>MEGPAGYLRRADVAQLTQELGTAFFQQQQLPAAMADTFLEHLCLLDIDSEPVAARSTSIIATIGPASRSVERLKEMIKAGMNIARLNFSHGSHEYHAESIANVREAVESFAGSPLSYRPVAIALDTKGPEIRTGILQGGPESEVELVKGSQVLVTVDPAFRTRGNANTVWVDYPNIVRVVPVGGRIYIDDGLISLVVQKIGPEGLVTQVENGGVLGSRKGVNLPGAQVDLPGLSEQDVRDLRFGVEHGVDIVFASFVRKA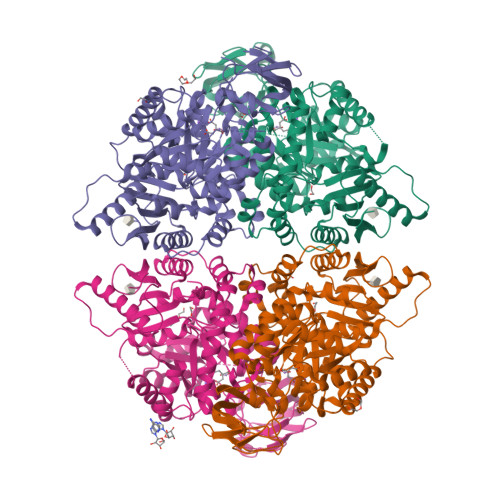SDVAAVRAALGPEGHGIKIISKIENHEGVKRFDEILEVSDGIMVARGDLGIEIPAEKVFLAQKMMIGRCNLAGKPVVCATQMLESMITKPRPTRAETSDVANAVLDGADCIMLSGETAKGNFPVEAVKMQHAIAREAEAAVYHRQLFEELRRAAPLSRDPTEVTAIGAVEAAFKCCAAAIIVLTTTGRSAQLLSRYRPRAAVIAVTRSAQAARQVHLCRGVFPLLYREPPEAIWADDVDRRVQFGIESGKLRGFLRVGDLVIVVTGWRPGSGYTNIMRVLSIS[4x]>[6x]MKCLFYIAGDVSNYSIVNYELNGQTQNTFFAAHALYNLFKPDKVIALIPDSLVKDNVSDEECYKNLVINRAKELNFAGMEEFMNKVEIRKIPNVGIASAIQCENGAPKKEKNKEGREVLKRLPYNEKRSPIFIFNAIYAIFKDEACDEYLVDLTHGTNVLVSIGMNVGALFNAKFYSAPVMGMPGKDSIVNIVELTDVVQATNDSLMIRSSIENLDERYFKDYSAKLSRLNPTIFEEEEKKVLTRVKGTDVNVVINFLWNIRNGFTVNAVKSMNELKNIINQLEEDLEKLKSFYKNWEEHKNFQGETLLVLSDLDSTLKVKDLLIEGNDLEKLNYLLDLYIKASIYDKALSLARELPVAICLNKVGGGMFDDKNEKYKHCNEIVTSYLRLRYSGLMEFRNTLMHGGLSTDMKPNVDKDGNITPGKIVTKNKIEDFVKRELRNYFDKIVNFLSSA

SisCsx1, as other members of the Csm6/Csx1 family, is composed of an N-terminal CRISPR-Cas-associated Rossmann Fold (CARF) domain connected to an α-helical higher eukaryotes and prokaryotes nucleotide-binding (HEPN) domain by a helix-turn-helix (HTH) domain. The SisCsx1 monomers are curled around the two-fold axis to form a dimer, and three of these dimers oligomerize through their HEPN domains into an equilateral trimer, thus assembling into a hexamer. Each dimer contains a cOA4 binding site at the vertex of the triangular assembly, and a catalytic pocket located 70 Å away inside the triangular oligomer along the two-fold dimer axis. We show that cOA4 binding activates a cooperative sequential catalytic response in a hexameric SisCsx1 complex and that the RNase activity is switched-off by Ring nucleases, which cleave cOA423.

To address that in the current study, we solved the atomic structures of SisCsx1 in its apo and cOA4 (cOA composed of 4 AMP units) bound forms. A SEC-MALLS analysis revealed that SisCsx1 is an oligomer of 300 kDa corresponding to a hexameric assembly. A cryoEM map of the complex at medium resolution was used as a model to solve the phase problem by molecular replacement in an apo SisCsx1 crystal belonging to the P21 space group. The SisCsx1 hexamer is built because of a split helical insertion (V365-N400) and the last helix at the C-terminus (D445-A454) in the HEPN domain. The α-helix spanning residues 375-391, establishes a series of contacts with the same segment in the adjacent monomer with the helices inversely oriented, and a well-conserved cysteine bridge (C361-C380) positions the hexamerization helix. The helices fit into each other and the central interaction surface is mainly hydrophobic. The hydrophobic interface is flanked by several polar interactions.> GSHMASPNGQTKPLPALKLALEYIVPAMNKHGICVVDDFLGKETGQQIGDEVRALHDTGKFTDGQLVSQKSDSSKDIRGDKITWIEGKEPGCETIGLLMSSMDDLICHCNGKLGSYKINGRTKAMVACYPGNGTGYVRHVDNCNGDGRCVTCIYYLNKDWDAKVSGGILRIFPEGKAQFADIEPKFDRLLFFWSDRRN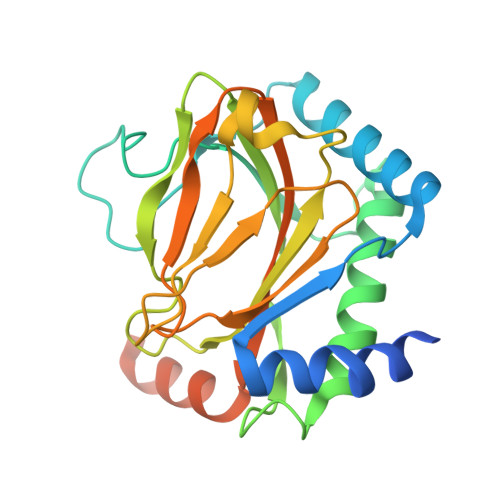PHEVQPAYATRYAITVWYFDADERAAAKVKYLTGEKGVRVELNKPSDSVGKDVF> MFRGIVQGRGVIRSISKSEDSQRHGIAFPEGMFQLVDVDTVMLVNGCSNTVVRILGDMVYFDIDQALGTTTFDGLKEGDQVNLEIHPKFGEVVGRGGLTGNIKGTALVAAIEENDAGFSVLIDIPKGLAENLTVKDDIGI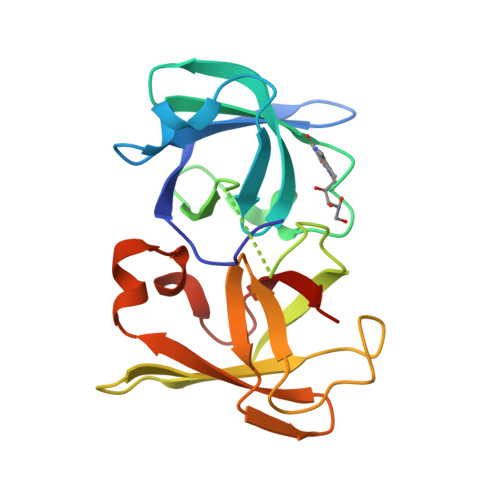DGISLPITDMSDSIITLNYSRDLLASTNIASLAKDVKVNVEILNEW> CCGC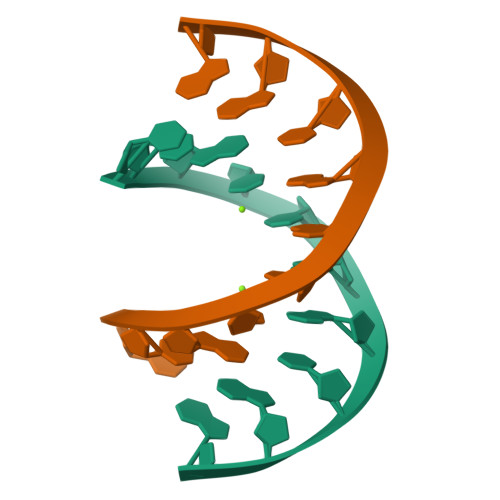CGGCGG> GPGSMSDKNFLVIDDNEVFAGTLARGLERRGYAVRQAHNKDEALKLAGAEKFEFITVDLHLGNDSGLSLIAPLCDLQPDARILVLTGYASIATAVQAVKDGADNYLAKPANVESILAALQTNASEVQAEEALENPVVLSVDRLEWEH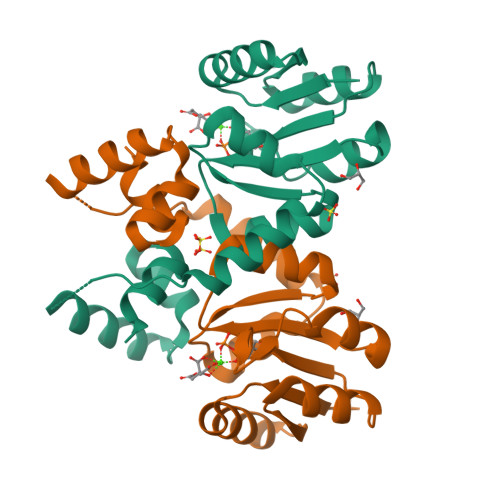IQRVLAENNNNISATARALNMHRRTLQRKLAKKPVRQ>MGFLSGKRILVTGVASKLSIAYGIAQAMHREGAELAFTYQNDKLKGRVEEFAAQLGSDIVLQCDVAEDASIDTMFAELGKVWPKFDGFVHSIGFAPGDQLDGDYVNAVTREGFKIAHDISSYS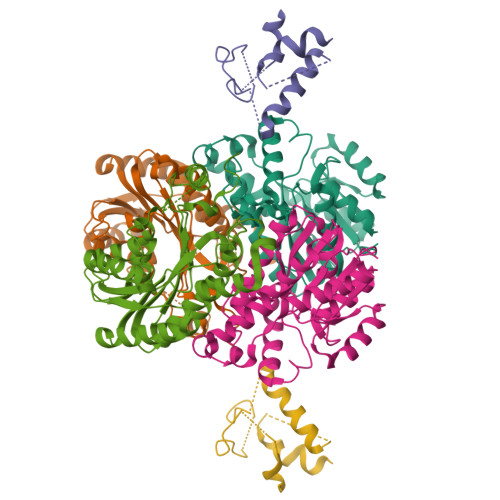FVAMAKACRSMLNPGSALLTLSYLGAERAIPNYNVMGLAKASLEANVRYMANAMGPEGVRVNAISAGPIRTLAASGIKDFRKMLAHCEAVTPIRRTVTIEDVGNSAAFLCSDLSAGISGEVVHVDGGFSIAAMNELELK[2x];> MSTIEERVKKIIGEQLGVKQEEVTNNASFVEDLGADSLDTVELVMALEEEFDTEIPDEEAEKITTVQAAIDYINGHQA>[2x]SFLPAAELEETPEALLLK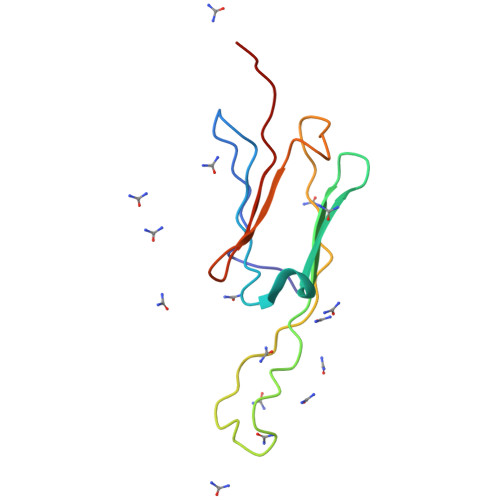VELPGMDPKDIDVQVTAEAVSISGERKSETKTETEGMKRTEFRYGKFQRVIPLPVRIQNTSVKAEYKDGILHLTLPKAEEE> ETGFPEDSEPISISHGNYTKQYPVFVGHKPGRNTTQRHRLDIQMIMIMNGTL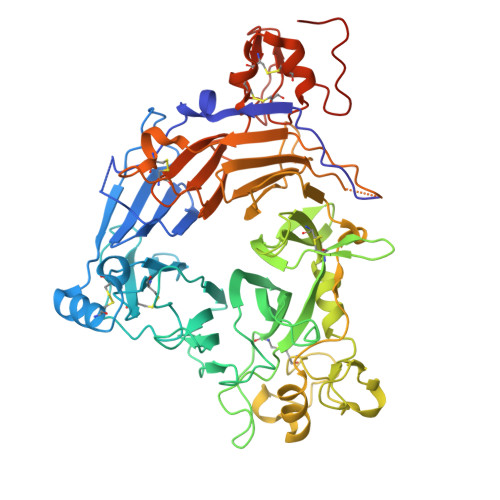YIAARDHIYTVDIDTSHTEEIYCSKKLTWKSRQADVDTCRMKGKHKDECHNFIKVLLKKNDDALFVCGTNAFNPSCRNYKMDTLEPFGDEFSGMARCPYDAKHANVALFADGKLYSATVTDFLAIDAVIYRSLGESPTLRTVKHDSKWLKEPYFVQAVDYGDYIYFFFREIAVEYNTMGKVVFPRVAQVCKNDMGGSQRVLEKQWTSFLKARLNCSVPGDSHFYFNILQAVTDVIRINGRDVVLATFSTPYNSIPGSAVCAYDMLDIASVFTGRFKEQKSPDSTWTPVPDERVPKPRPGCCAGSSSLERYATSNEFPDDTLNFIKTHPLMDEAVPSIFNRPWFLRTMVRYRLTKIAVDTAAGPYQNHTVVFLGSEKGIILKFLARIGNSGFLNDSLFLEEMSVYNSEKCSYDGVEDKRIMGMQLDRASSSLYVAFSTCVIKVPLGRCERYGKCKKTCIASRDPYCGWIKEGGACSHLSPNSRLTFEQDIERGNTDGLGDCHNGSWSHPQFEK>GSDELKWNKGYSLPNLLEVTDQQKELSQWTLGDKVKLEEGRFVLTPGKNTKGSLWLKPEYSIKDAMTIEWTFRSFGFRGSTKGGLAFWLKQGNEGDSTELFGGSSKKFNGLMILLRLDDKLGESVTAFLNDGTKDLDIESSPYFASCLFQYQDSMVPSTLRLTYNPLDNHLLKLQMDNRVCF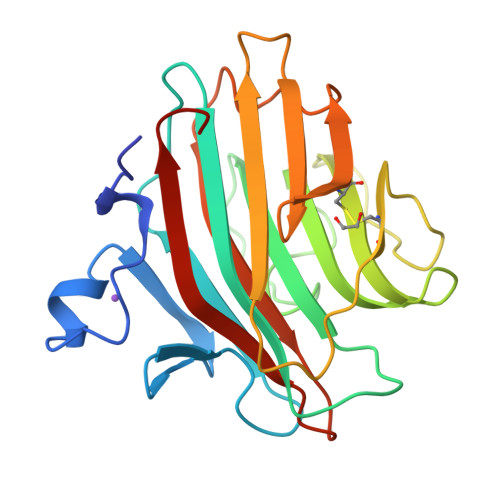QTRKVKFMGSSPFRIGTSAINDASKESFEILKMKLYDGVIEDSL[2x]Staphylococcal enterotoxin B (SEB) is one of seven toxins secreted by Staphylococcus aureus, and is classified as a bacterial superantigen. SEB is one of the group II superantigens, a group that includes SEC and SpeA. Superantigens in this group bind to T-cell receptors (TCRs) in a peptide-independent manner to generate an abrupt and strong immune response. This 28 kDa toxin consists of two domains, domain I (amino acids 30–120) and domain II (amino acids 127–239), which are composed of a β-barrel structure and antiparallel β-sheets, respectively.

We designed a vaccine candidate, S19, with reduced TCB–SEB interaction by introducing the following four mutations: N23A, Y90A, R110A and F177A. S19 was originally designed to make fewer molecular interactions with TCB than wild-type SEB, as a result of the removal of key interacting side chains. S19 maintained a similar overall structure to SEB, which is required for its antigenicity as a vaccine candidate. However, S19 exhibits some structural changes in its flexible-loop region (Tyr94–Thr113; Benedik et al., 2014). Although the entire structure of the loop region has not been determined, owing to its outwards orientation and high flexibility, the N-terminal region of this loop is well stabilized by intramolecular hydrogen bonds and by a disulfide bridge between Cys93 and Cys113. The Y90A mutation was the sole reason for the observed structural change, as depicted in Fig. 1(c). Tyr91 of S19 moved into the original position of Tyr90, which had been stabilized by hydrogen bonds to Asn60 and Asn88. The disulfide bridge in SEB was broken in S19 owing to the ∼8 Å translocation of Cys93 in S19. The interface areas between TCB and SEB and between MHC and SEB were decreased 27 or 14% by the mutations, respectively; thus, the simulation reflected the loss of binding residues. The number of simulated hydrogen bonds also decreased from 10/10 to 8/5, respectively. S19 was originally designed to have a lower binding affinity for TCB, but structural determination revealed reduced interactions with both binding partners, TCB and MHC.

>SQPDPKPDELHKSSKFTGLMEAMKVLYDDNHVSAINVKSIDQFLYFDLIYSIKDTKLGNYDNVRVEFKNKDLADKYKDKYVDVFGANYAYQCYFSKKTNDINSHQTDKAKTCMYGGVTEHNGNQLDKYRSITVRVFEDGKNLLSFDVQTNKKKVTAQELDYLTRHYLVKNKKLYEANNSPYETGYIKFIENENSFWYDMMPAPGDKFDQSKYLMMYNDNKMVDSKDVKIEVYLTT[2x]>SSRLVTETQYGTMLMRTADWVSTAPFDGHMSVFPVGTERTMRGQVAEYQQAMTKWQTKYHTLSIEEHGAFGGLSGQTSNEKGLSVMALSQHDSEPYLSQHKDNGAPAVNTADVVSFITERYATTAEVKAALDNGEFQIAWASAP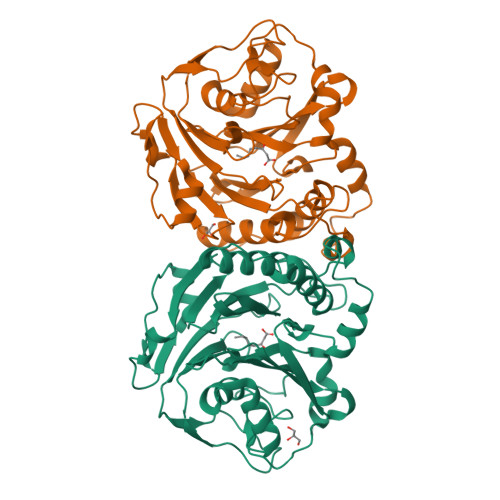NGMEHAAPLHYSVVDADGNIMLIQLVKGGEQKIYLGDAESDLRVKTNDPLQEKHREYMQQFDLKDPSVATKMPWSIGGLERNSRLLAMSTHMDLEGLSYTETVARQKGTFDAAALVPFGVQDPKTGEDYPSFFSMQYNLDNGDIWFRSLMSGKEIKFNLEDTKQFKTPMHADIMAQVDKGAQTITWSKMHHHHHH[2x]>[3x]GPLGSMKPINIQDQFLNQIRKENTYVTVFLLNGFQ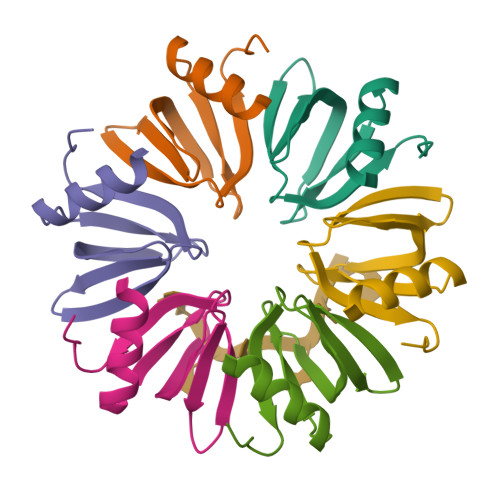LRGQVKGFDNFTVLLESEGKQQLIYKHAISTFAPQKNVQLELE>SQQEFLERARQYLEEARRDLTTRPYYYYVGSDSDGTTREARSREEYAKPETQEFEKRVRSLIEELKNSEDKENYEIYETDYSWTETENGETRTHHIYFAYVKKDGKLEALLLRIESSGPLT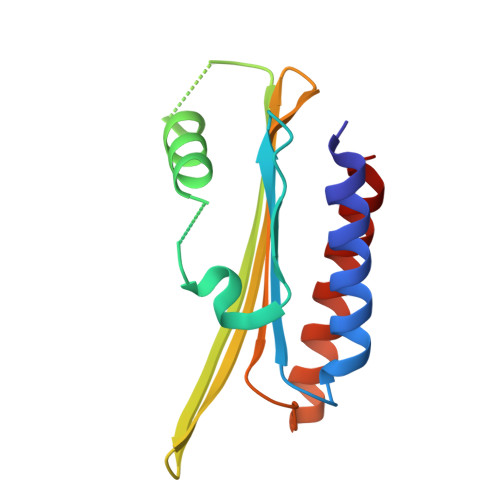DEETIEKTTRLLDEIYEKLESLS[4x]> SKM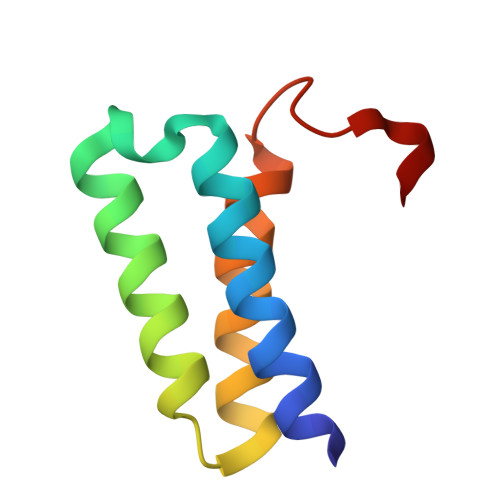SDVKCTSVVLLSVLQQLRVESSSKLWAQCVQLHNDILLAKDTTEAFEKMVSLLSVLLSMQGAVDINKL> NLLAGDTKEQRILNHVLQHAEPGNAQSVLEAIDTYCEQKEWAMNVGDKKGK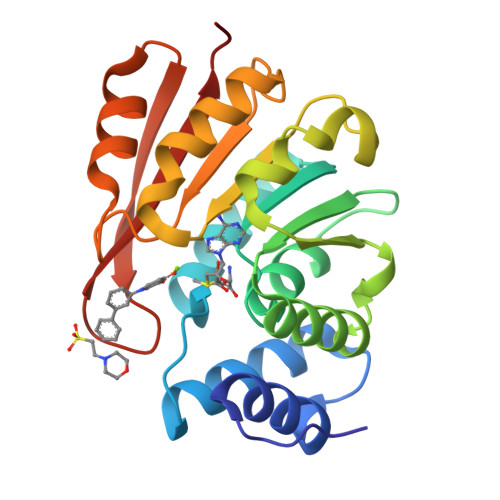IVDAVIQEHQPSVLLELGAYCGYSAVRMARLLSPGARLITIEINPDCAAITQRMVDFAGVKDKVTLVVGASQDIIPQLKKKYDVDTLDMVFLDHWKDRYLPDTLLLEECGLLRKGTVLLADNVICPGAPDFLAHVRGSSCFECTHYQSFLEYREVVDGLEKAIYKGP>[2x]MLAILYDRIRPDERMLFERAEALGLPYKKVYVPALPMVLGERPEALEGVTVALERCVSQSRGLAAARYLTALGIPVVNRPEVIEACGDKWATSVALAKAGLPQPKTALATDREEALRLMEAFGYPVVLKPVIGSWGRLLAKVTDRAAAEALLEHKEVLGGFQHQL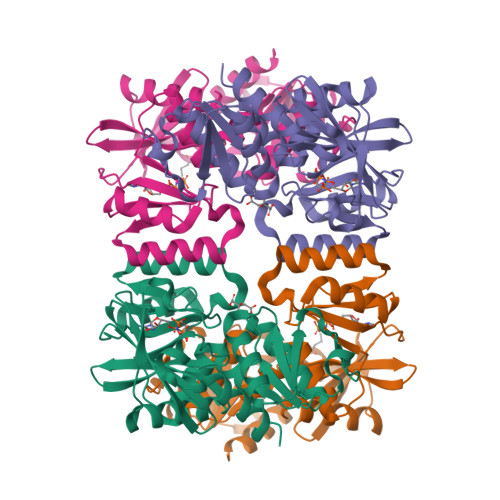FYIQEYVEKPGRDIRVFVVGERAIAAIYRRSAHWITNTARGGQAENCPLTEEIARLSVGAAEAVGGGVVAVDLFESERGLLVNEVNHTMEFKNSVHTTGVDIPGEILRYAWEVARG>[4x]GPGSMTDYIRDGQAIYDRSFAIIRAEADLRHIPADLEKLAVRVIHACGMVDVANDLAFSEGAGKAGRNALLAGAPILCDARMVAEGITRSRLPAD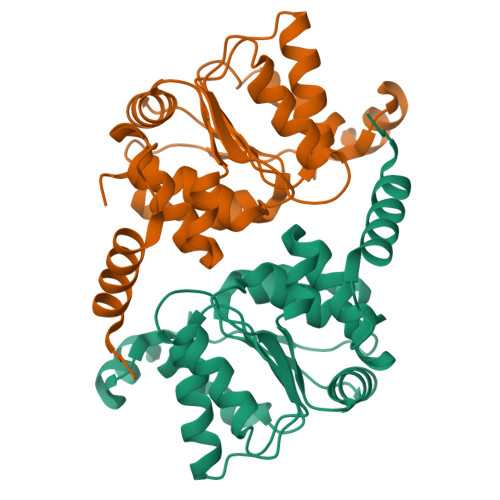NRVIYTLSDPSVPELAKKIGNTRSAAALDLWLPHIEGSIVAIGNAPTALFRLFELLDAGAPKPALIIGMPVGFVGAAESKDELAANSRGVPYVIVRGRRGGSAMTAAAVNALASERE(1S)-1-(3,4-DICHLOROPHENYL)-3-[FORMYL(HYDROXY)AMINO]PROPYL}PHOSPHONIC 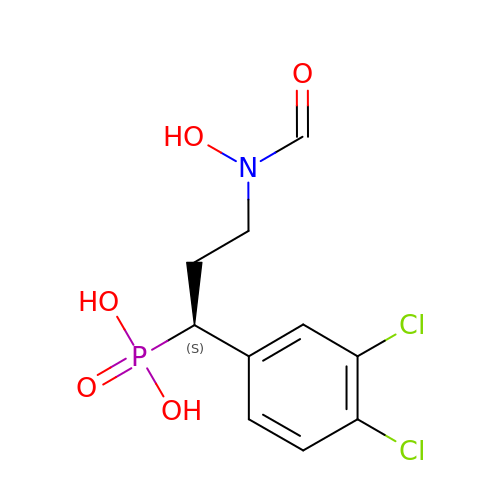ACID | C10 H12 Cl2 N O5 P | AJGPMMOCRYQLNY-JTQLQIEISA-N> LGKFSQTCYNSAIQGSVLTSTCERTNGGYNTSSIDLNSVIENVDGSLKWQPSNFIETCRNTQLAGSS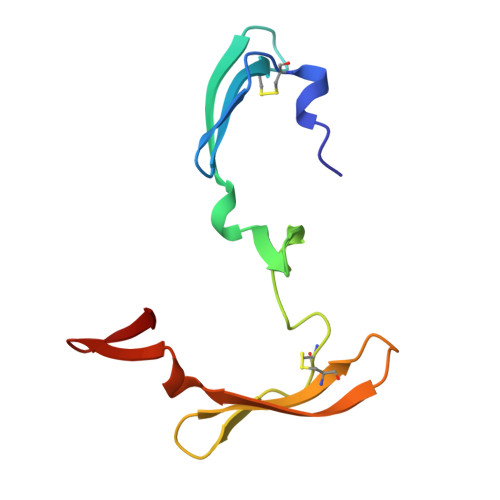ELAAECKTRAQQFVSTKINLDDHIANIDGTLKYE>[4x]GSRQIVD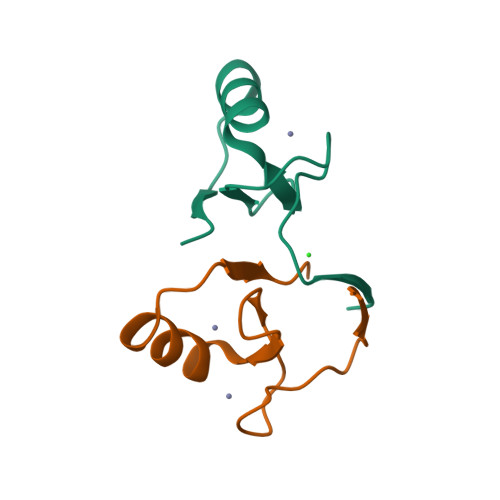AQAVCTRCKESADFWCFECEQLLCAKCFEAHQWFLKHEARPLAE> MGSSHHHHHHSSENLYFQGHMASAMSSPTRALGFLYSCYGGVSTDLPSAYLGEINSTTDEYVLPYSWNTDGYWGAYAFNTASSTNQDWLWGTTYQYIG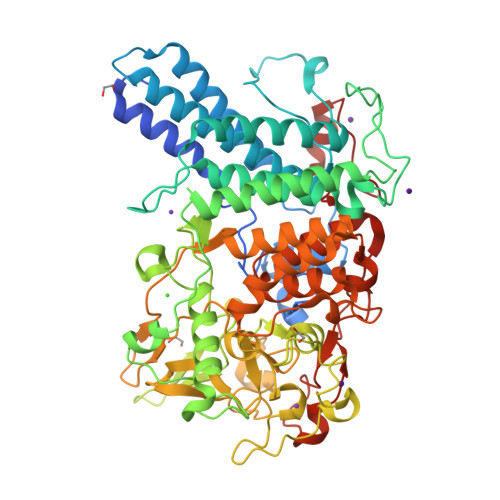QCYLFLQKLENAGSDIASDAEKEQWRAECQFLVAYYHFATLRRYGPIPITDSYIPMDTPTSEYNGRFHFDYCVDWIANQLDEAAKVLPANRTATNEWGRATSTIAKAVKARLLLYAASPLWNGSFPYPNWQNENFETPGYGKALVSNTYDKSKWERALAACQEALTLATTSGDRELYDDDEYYSRQSLNLPFVPGVADVEDNKEFLKNVMKMRYAVSTRESEGNKEIIWGLSNQFDFYSRYPLRILKKSDGTWHAGYSGVSPTLYTFEHFYTANGKLPEKDLDFTPSSEWFESAGISSREDIIKLNVGREPRFYAWMAFDGGDYGTKFAAGSPLKLEMRNSEMHGYNPSLFNRDHSVTGFLTQKFVDPVTEFYTAGGSTSGTSAPTILFRLAELYLNVAECHAALGNTQEAIDALNPVRERAGIPKLTLADITNNMTIKDWVHNERFVELWNEGHRFFDVRRWAEGAKYFGANKREGLNAEVQSPTFEEFNKRTTVDAPYVWENRMYLNPVFYNEVYKNPQMVQAPGY>[2x]MQKEPRKVREFRRREQEILDTALKLFLEQGE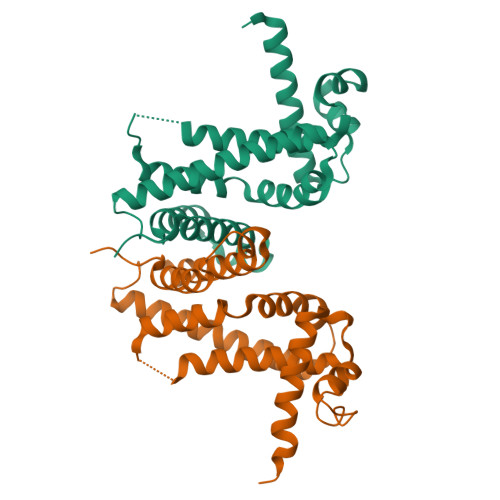DSVTVEMIADAVGIGKGTIYKHFKSKAEIYLRLMLDYERDLAALFHSEDVARDKEALSRAYFEFRMRDPQRYRLFDRLEEKVVKTSQVPEMVEELHKIRASNFERLTQLIKERIADGKLENVPPYFHYCAAWALVHGAVALYHSPFWREVLEDQEGFFHFLMDIGVRMGNKRKREGDAPSA> GDTKEQRILNHVLQHAEPGNAQSVLEAIDTYCEQKEWAMNVGDKKGKIVDAVIQEHQPSVLLELG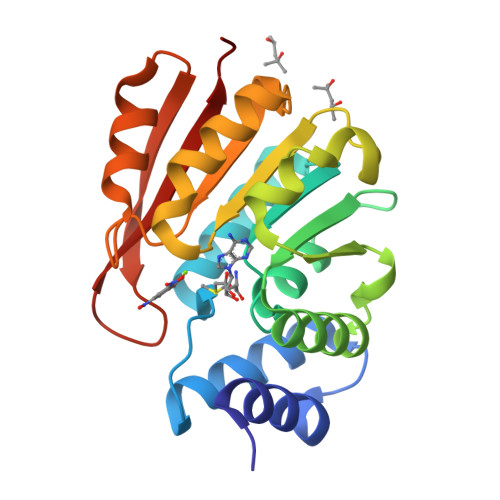AYCGYSAVRMARLLSPGARLITIEINPDCAAITQRMVDFAGMKDKVTLVVGASQDIIPQLKKKYDVDTLDMVFLDHWKDRYLPDTLLLEECGLLRKGTVLLADNVICPGAPDFLAHVRGSSCFECTHYQSFLEYREVVDGLEKAIYKGP(2S)-2-[4-(aminomethyl)benzyl]-3-[(R)-[(1R)-1-amino-3-phenylpropyl](hydroxy)phosphoryl]propanoic 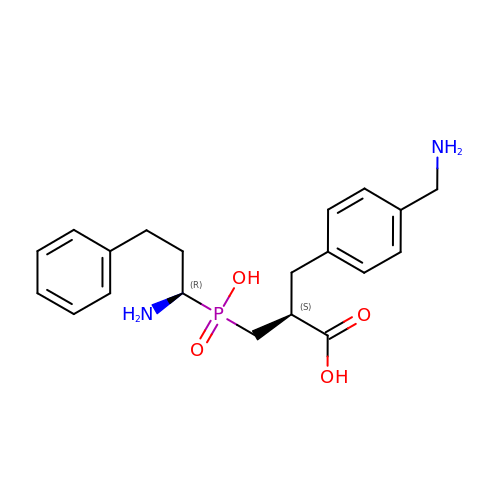acid | C20 H27 N2 O4 P | XZFPYKBNMOQQLL-RTBURBONSA-N2-(hydroxymethyl)phenyl 6-O-phosphono-beta-D-glucopyranoside 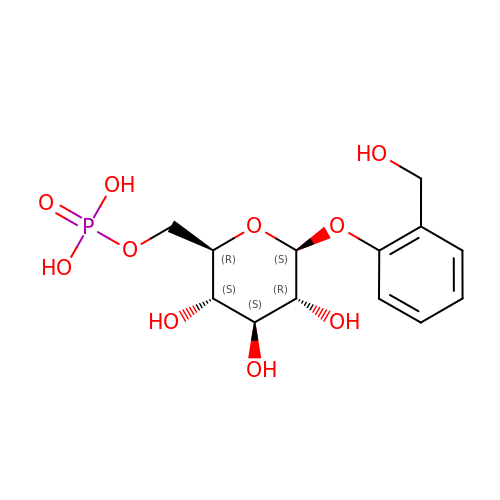| C13 H19 O10 P | FSJKOMDYZYBBLV-UJPOAAIJSA-N> ERVNVNLTSIKKLREKVDDSIHRELTDIFANLNYVGVVDEERRLAAIQHDLKLFLIDYGSVCYELFYQIGLTDFANFGKINLQSTNVSDDIVLYNLLSEFDELNDDASKEKIISKIWDMSSMLNEYYSIELVNDGLDNDLKSVKLKSLPLLLKGYIPSLVKLPFFIYRLGKEVDWEDEQECLDGILREIALLYIPDMVPKVDTSDASLSEDEKAQFINRKEHIS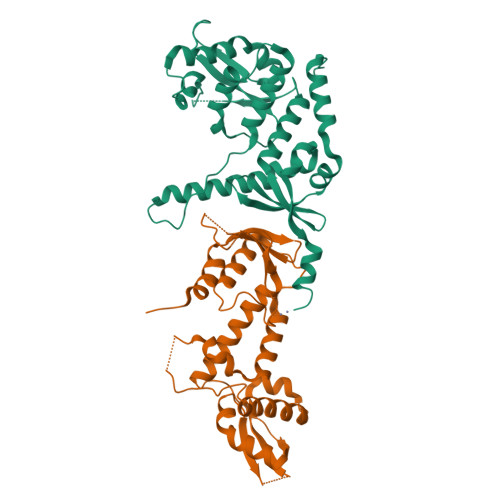SLLEHVLFPCIKRRFLAPRHILKDVVEIANLPDLYKVFERC;> GKTITDFSISRSVLAKYEVINQVDKKFILIRCLDQSIHNCPLLVLVDQHACDERIRLEELFYSLLTEVVTGTFVARDLKDCCIEVDRTEADLFKHYQSEFKKWGIGYETIEGTMETSLLEIKTLPEMLTSKYNGDKDYLKMVLLQHAHDLKDFKKLPMDLSHFENYTSVDKLYWWKYSSCVPTVFHEILNSKACRSAVMFGDELTRQECIILISKLSRCHNPFECAHGRPSMVPIAEL The Portal Protein (PP) complex is a central component of Caudovirales virions in the process of self-assembly of phages. The PP has multiple functions: (1) as a nucleation point for capsid formation; (2) as part of the motor for loading the genome into the capsid; (3) as a head-full sensor; and (4) as a conduit for genome translocation. All portal protein primary structures are characterised by a common fold comprising four conserved domains: The capsid-facing C-terminal crown, the interior wing and stem, and the tail-facing clip domains. Using cryoEM, we determined the structures of two portal proteins: GA1 gp10, and phiCPV4 gp17, which are phages of the Salasmaviridae and Guelinviridae families respectively. Both GA1 gp10 and phiCPV4 gp17 PPs have the canonical fold and domain organisation found in the portal protein phi29 gp10.

The phiCPV4 phage belongs to the Guelinviridae family and infects Clostridium perfringens, a pathogenic scourge of the poultry industry, which causes foodborne illnesses in humans. Guelinviridae infecting Clostridium species also cluster together (in yellow) with the phiCPV4 PP (gp17) sharing 28.7% sequence identity with phi29 gp10. The height and diameter the phiCPV4 gp17 dodecamer are 82 Å and 158Å. In phiCPV4 gp17 the N-terminus could be traced from residue Val23 and forms the α1 helix similar to that of phi29 gp10 and GA1 gp10. Likewise, monomers of phiCPV4 gp17 are held together by 4 hydrogen bonds between the α3 helices: Gln152A, Tyr145A, Lys165B, Asn158B, where A and B designate adjacent subunits. Interestingly, in phiCPV4 gp17 the β-sheet of the clip is formed by three strands β8, β9, and β10 of the same subunit. In phiCPV4 the inter-monomeric interactions occur between α4 (Asn176B, Met180B, Leu183B, Tyr184B) and β9 (Leu195A, Val196A, Glu198A) of the adjacent subunit. The insertion of the Lys-Leu-Ala-Glu-Ala motif (residues 197–202 forming helix α4′) followed by the loop Gln-Ala-Leu-Gln-Glu, makes the link between β9 and β10 bigger, allowing them to form a common β-layer. The inter-monomeric interactions are located between β9 and α4 in phiCPV4 gp17, which is different from all other PPs; while in phi29 and GA1 gp10 it is the β8 and β9 from adjacent subunits that make the more typical inter-monomeric interactions. This is an unexpected observation, since all other Caudovirales PPs described to date have the β-sheet of the clip domain formed by strands from adjacent subunits.

>[12x]MSKRKSYWNQGDKILLKNDVFMVDRYYDYYSNMGLNRFRWKNLPPGMESRHIEQALFNEGQAVFFKNTDPNEPYGFLCLPCAPSNGQNIYGDPVDFNGIGVNKYFTNLSPLNAVRILDNDNGLAPVRHIAYYTYLMSQIEMTINMNLDQQKFPIIIGATQKNKLSMENLYEKYSSFEPNILVDEKLAQALQEGKGFDALNTQAPYLLDKLADFKKTCENELLTFLGINNTNNDKRERLLTDEVNANNSQITFVLEMAYKNRLDACKRINEMFGLNLEVEKVVNLLEVDMKGDVKNEGINGE~{N},~{N}-dimethyl-1-[1-[2-(1-methylindol-4-yl)-3~{H}-imidazo[4,5-b]pyridin-7-yl]pyrazol-4-yl]methanamine 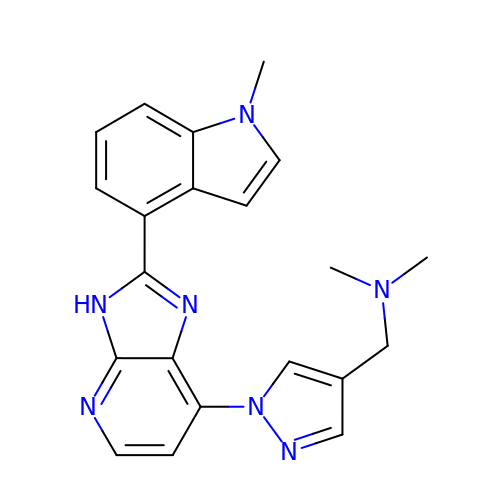| C21 H21 N7 | TVDTXKARIOKJSV-UHFFFAOYSA-N> MGSSHHHHHHSSGLVPRGSHAMADYTEQDAMRVQAVKTYIDNVLQEGRSQIKTTPLLADGINTTTRKPVEWIYPDGRTATISNFANQQNFLRALTAMSVVTEDQRYQLEAVRITRYFMDNFIADNGLFYWGGHRFVNLDTLELEGPQNKNSVHELKNHYPYYPFLYHVDPHATERYIKAFWQAHVEDWQSLDMGRHGSYSKNYDDKVFHRPIPASLVDQSKLPIMPETKGLTFINAGSDLIYAAYQLDWLAPSANAQGSAAWGQYLMTQYKLAKHPKTGAPVYQFTSPKKREWPPQSDKDTNSKYGDRAARQFGPELGNIAREGNVLFKSNDKSIVFNNALIELHLAEQRNDAAIREQVVDALLNFYRLAYNPENGTIKPIFSDGTSIEGIPLARDGYYGPKGRVFNAHKPKTEEYLLPILRAYRLQADPELWQLAANMTHHYGWGSLGNDAKAKPTLNMQLSSVSPMTLFSAIELYQITQQPEYLEFARAAADKLVEKRFVRGYFLAN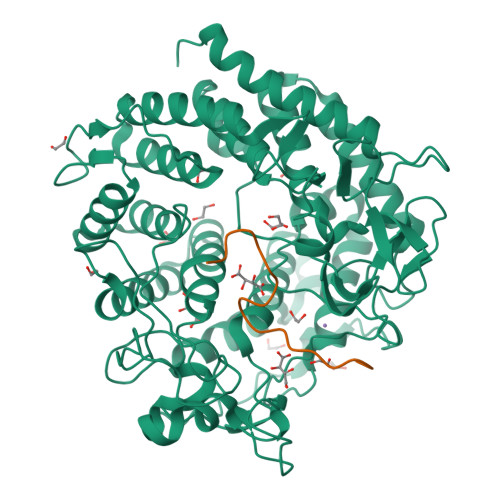PRYLNASIDAIEPLALLTLDATLKGKTAQVAPYLSGSGYIHGEFAGKENAYDTNEIYKQTR;> HHHHHHHSSGLVPRGSHA>GSSGAFEDRDPTQFEERHLKFLQQLGKGNFGSVEMCRYDPLQDNTGEVVAVKKLQHSTEEHLRDFEREIEILKSLQHDNIVKYKGVCYSAGRRNLKLIMEYLPYGSLRDYLQKHKERIDHIKLLQYTSQICKGMEYLGTKRYIHRDLATRNILVENENRVKIGDFGLTKVLPQDKEYYKVKEPGESPIFWYAPESLTESKFSVASDVWSFGVVLY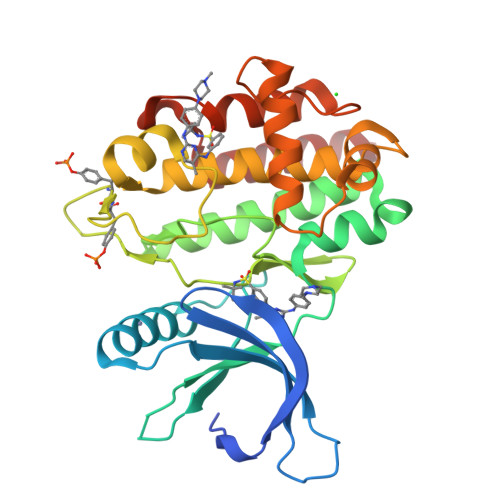ELFTYIEKSKSAPAEFMRMIGNDKQGQMIVFHLIELLKNNGRLPRPDGCPDEIYMIMTECWNNNVNQRPSFRDLALRVDQIRDNMAG[4x]8-oxa-2-azaspiro[4.5]decan-2-yl-[2-[(3~{S})-3-oxidanylpyrrolidin-1-yl]-1,3-thiazol-5-yl]methanone 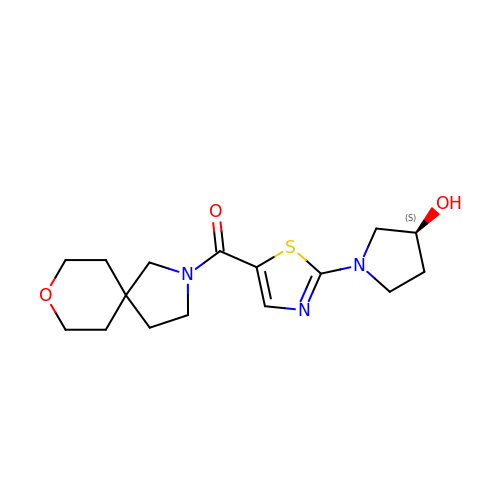| C16 H23 N3 O3 S | PDHLSHPRWHXZMR-LBPRGKRZSA-N> MSKAEMVANKIKERFPNAEVVVKTNKWGRERVWVRISREEYKELMKFIRELDPEAHYSIGIEQDWGDELGFLNHILLFYDEPPGVSLLIDVHAPKDNPVLPDTSDIFPISLQFEREGMEMVGLDFEGAPDKRRLFLPDDFPEGIYPLRTDEKGVPEEMVKNAGHP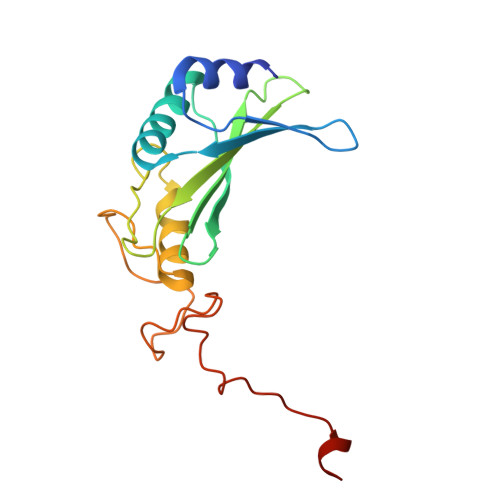YLLRREKK(2R)-3-(Benzylsulfanyl)-2-({[(4-methylphenyl)methyl] [(4 phenylphenyl)carbonyl] carbamoyl}amino) 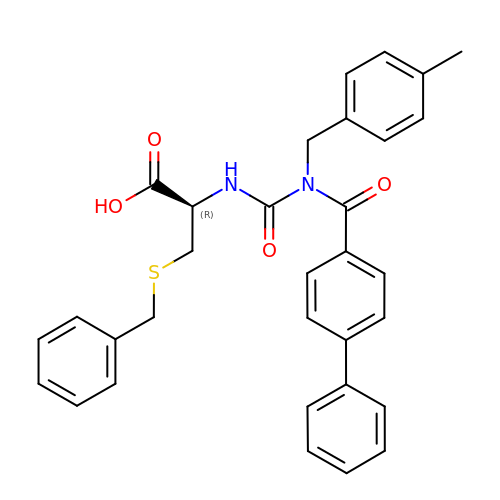propanoic acid  | C32 H30 N2 O4 S | DCCZUUDOXXRWAG-LJAQVGFWSA-N>GSFKFTAQQHVYDINGVKVGGQPGEYPTVLIGSIFYRGHKIVSDGQKGIFDKDAAKALLDQEAELSAETGNPFIIDVLGESVEALTKYVEFILENTTAPFLLDSISPDVRVGALKNLGKDPEIQKRLIYNSIEEHYTEEELAAIKEAGLKTAVILAFSKKALKPNARIDLLQGKDDKEGLIAAAKRAGIEQFLVDPGVLDVASNSWTTEAINVVKEQFGYPGGCAPSAAVYLWKKMRSKGTPFFEVAGAAVFTYPITQGADFILYGPMMNAPWVYRAIATTDAMIAYNNKLTGVKMGTTEHPLLKIF[2x]

During energy production in Desulfitobacterium hafniense, MtgA catalyzes the methyl transfer from methylcobalamin (Cbl‐CH3) to THF in the catabolism of glycine betaine (GB). Despite its lack of sequence identity with known structures, we could show that MtgA forms a homodimeric complex of two TIM barrels. The topology of each subunit is characterized by a funnel of eight parallel β‐sheets connected by α‐helices on the outside that form a complex of two perpendicularly oriented TIM barrels. The active‐site cavity is located inside the hydrophilic core of each barrel.

Apart from snapshots of individual reaction steps of MtgA, structure‐based mutagenesis combined with enzymatic activity assays allowed a mechanistic description of the methyl transfer between Cbl‐CH3 and THF.>[2x]HHHHHHGSERTGTQPLGVQGLTEEQRMMIRELMDAQMKTFDTTFSHFKNFRLPGVLSSGCELPESLQAPSREEAAKWSQVRKDLCSLKVSLQLRGEDGSVWNYKPPADSGGKEIFSLLPHMADMSTYMFKGIISFAKVISYFRDLPIEDQISLLKGAAFELCQLRFNTVFNAETGTWECGRLSYCLEDTAGGFQQLLLEPMLKFHYMLKKLQLHEEEYVLMQAISLFSPDRPGVLQHRVVDQLQEQFAITLKSYIECNRPQPAHRFLFLKIMAMLTELRSINAQHTQRLLRIQDIHPFATPLMQELFGITGSSGGSGGSSHSSLTERHKILHRLLQEGSPSDITTLSVEPD

PXR is a nuclear receptor that can be activated by diverse compounds to elevate metabolism, negatively impacting drug efficacy and safety. As a xenobiotic sensor, PXR is activated by structurally diverse compounds and plays a major role in drug metabolism and drug-drug interactions by regulating transcription of genes encoding drug metabolizing enzymes, drug conjugating enzymes, and drug transporters. Here, we report structurally related PXR-selective agonists and antagonists and their corresponding co-crystal structures to describe mechanisms of antagonism and selectivity. Structural and computational approaches show that antagonists induce PXR conformational changes incompatible with transcriptional coactivator recruitment.

In all reported PXR LBD structures, there is no difference in α12 conformation regardless of the presence or absence of ligand; indeed, most NR structures display the same α12 conformation. The observation that ligand binding does not affect α12 conformation in crystal studies provided us with the opportunity to determine differences in interactions between agonists and antagonists to residues of the PXR ligand binding pocket under similar structural circumstances.>GPKITLLTLIKTAEHWARQDIRTIEDSKLRALLTLCAVMTRKFSKSQLSLLCETHLRREGLGQDQAEPVLEVYQRLHSDKGGSFEAALWQQWDRQSLIMFITAFLNIALQLPCESSAVVVSGLRTLVPQ[4x];>PTVAPPAPVYR[4x]

Viral protein 30 (VP30) proteins are present in all filoviruses and perform several important functions, but homologues are lacking in other negative-sense RNA viruses. Additionally, VP30 binds RNA in the presence of zinc and associates with the viral RNA synthesis machinery, which includes nucleoprotein (NP), VP35, and large (L) protein that contains the enzymatic activities. EBOV VP30 (eVP30) is critical for viral transcription (mRNA synthesis), because it is required for initiation at EBOV NP (eNP), the first gene of the seven gene genome. eVP30 has also been implicated in regulation of co-transcriptional editing of viral glycoprotein mRNAs and in modulation of viral transcription reinitiation. We demonstrate that eVP30 binds directly to eNP.

We generated protein crystals for structure determination using the purified eVP30110–272/eNP600–739 complex. Initial low-resolution diffracting crystals were optimized by in situ proteolysis and resulted in several well-diffracting crystals. In contrast to eVP30/eNP contacts, which are largely similar even though the structures belong to different asymmetric units, the ternary configurations of eVP30 suggest that the eVP30/eNP interaction may not impact eVP30–eVP30 interactions. Residues from eNP that span 600–612 are highly conserved not only across all ebolavirus genus members but also marburgvirus as well. Although PPXP motifs typically form a left-handed turn, in the eNP/eVP30 complex structures, the conformation of this motif does not form the expected polyproline type II helix. Instead, these highly conserved eNP residues make extensive contacts with eVP30 residues in an extended conformation. Although the binding pocket is somewhat shallow, the interaction site displays a shape complementarity (Sc) score of 0.6, which is considered significant. Analysis of the interface reveals that there are seven hydrogen bonds between eVP30 and eNP and a number of hydrophobic contacts, which make up much of the observed total of 1,923 Å2 buried surface area. For example, eVP30 Q203A or R213A or Q229A did not result in loss of binding to eNP WT in the FPA, whereas eVP30 E197A and W230A resulted in a near complete loss of binding. However, our data show that the binding site identified in our structure, which includes residues such as W230, results in complete loss of binding and corresponding loss of activity in viral RNA synthesis.>DNVITRVVAVRNVSVRELSPLLRQLIDNAGAGNVVHYDPANIILITGRAAVVNRLAEIIKRVDQAGNREIEVVELGNASAAEMVRIVDALNRTTDAKNTPEFLQPKLVADERTNSILISGDPKVRDRLKRLIRQLDVEMASKGNNRVVYLKYAKAEDLVDVLKGVSDNLQAEKNSGQKGASSQRNDVVIAAHQGTNSLVLTAPPDIMLALQEVITQLDIRRAQV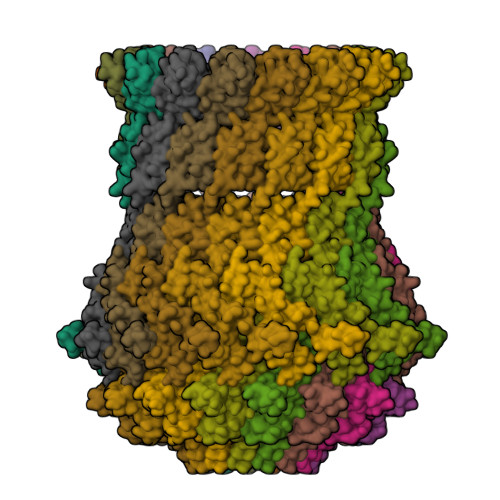LIEALIVEMAEGDGVNLGVQWGNLETGAVIQYSNTGTPIGKVMVGLEEAKDKTVTDSRWNSDTDKYEPYSRTEAGDYSTLAAALAGVNGAAMSLVMGDWTALISAVSSDSNSNILSSPSITVMDNGEASFIVGEEVPVITGSTAGSNNDNPFQTVDRKEVGIKLKVVPQINEGDSVQLNIEQEVSNVLGANGAVDVRFAKRQLNTSVIVQDGQMLVLGGLIDERALESESKVPLLGDIPILGHLFKSTNTQVEKKNLMVFIKPTIIRDGMTADGITQRKYNYIRAEQLYKAEQGLKLMDDGHIPVLPKFGEDKRHPAEIQAFIDQMEQQ[15x]>SNAAGFAQASPSAPVAGKDFEVMKSPQPVSAPAGKVEVIEFFWYGCPHCYEFEPTIEAWVKKQGDKIAFKRVPVAFRDDFVPHSKLFYALAALGVSEKVTPAVFNAIHKEKNYLLTPQAQADFLATQGVDKKKFLDAYNSFSVQGQVKQSAELLKNYNIDGVPTIVVQGKYKTGPAYTNSLEGTAQVLDFLVKQVQDKKL[4x]

Disulfide-bond-forming protein A (DsbA) catalyzes the formation of the disulfide bonds necessary for the activity and stability of multiple substrate proteins, including many virulence factors. DsbA works in tandem with its membrane-embedded partner protein DsbB, which is required to maintain DsbA in its active, oxidized state. B. pseudomallei is a Gram-negative bacterium that is found predominantly in tropical areas and is the causative agent of the deadly disease melioidosis. Binding was characterized using NMR and X-ray crystallo­graphy. Both 1 and 2 bind to a transient (or ‘cryptic’) pocket on BpsDsbA located adjacent to the redox active site which is not observed in the apo BpsDsbA structure.

Oxidized BpsDsbA was co-crystallized with 2 in a crystallization solution that typically generated crystals of the apoprotein, that is 200 mM Li2SO4, 100 mM HEPES pH 7.5, 29.5% PEG 3350. A crystal was harvested and diffracted to a resolution of 2.3 Å with space group P21 and unit-cell parameters a = 69.4, b = 59.4 , c = 105.4 Å, α = γ = 90, β = 104.9°. As such they were modelled as alternative conformations of the same molecule (with occupancies of 0.43 and 0.31). Similarly, we modelled Arg74 of chain B (Arg74-B) with two conformations which differ depending on the presence or absence of fragment 2 in orientation B (binding near the Tyr110 side chain of chain B). The two orientations A and B of fragment 2 sit in an almost completely closed pocket at the interface of protein chains A and B.> SAVSIPINNAGFENPFMDVVDDYTIDTPPGWTTYDPNNLVPEKRTTWTSNNGVGYVGPGTQFYNQLAPEGRNIGYIYLSQNPGSGVAGFEQCLDATLEPDTKYTLTVDVGALAGTFKGLSFAGFPGYRV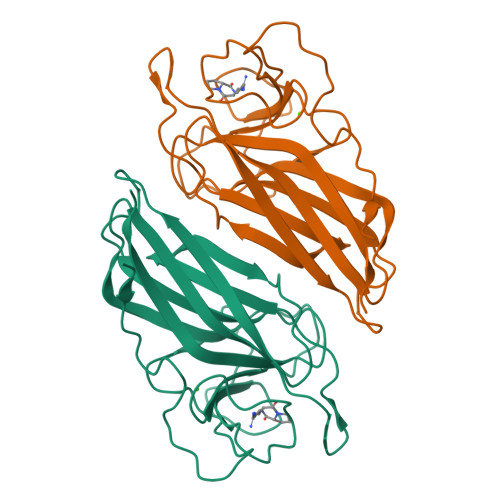ELLAGDTVLAADHNNLFIKEGEFKTSTVTYTSTAKDLHLGQKLGIRLVNLLQDKFSGLDFDNVRLTTEPTE Among the most important sources of epigenetic silencing in humans is the Human Silencing Hub (HUSH) complex, consisting of three proteins: Periphilin, TASOR and MPP8 (11). In the current model of HUSH-dependent repression HUSH spreads histone H3 lysine 9 trimethylation (H3K9me3), a transcriptionally repressive mark, by recruiting the H3K9 methyltransferase SETDB1 and its stabilizing factor ATF7IP to existing H3K9me3 marks via MPP8, which binds both H3K9me3 and ATF7IP. Here, we report the crystal structure of a Periphilin-TASOR minimal core complex and identify the key physicochemical properties of Periphilin necessary for HUSH complex assembly and epigenetic silencing. The Periphilin C-terminal region directs HUSH complex assembly by dimerizing and binding a single TASOR molecule through α-helical coiled-coil interactions.

Thus, a crystal structure of a Periphilin fragment spanning residues 292–367 bound to a TASOR fragment spanning residues 1014–1095 was determined using the single anomalous dispersion (SAD) phasing method, with bromine as the anomalous scatterer. The structure contains two Periphilin molecules and a single TASOR molecule. The Periphilin fragments form helical hairpins with a mixture of α-helix and 310-helix secondary structure. The two Periphilin hairpins pack against each other via a 118 Å2 hydrophobic interface formed by the hydrophobic side chains of Leu326, Leu333 and Ile337. The resulting Periphilin homodimer has twofold symmetry. The TASOR molecule forms two α-helices that wrap around the outer surfaces of the Periphilin dimer. The TASOR helices add a third helix to each Periphilin helical hairpin to form two three-helix coiled-coils. Unusually, however, each Periphilin subunit binds to a different TASOR sequence (residues 1014–1052 and 1072–1093, respectively) with an identical binding surface. Notably residues 1055–1071 of TASOR, between the two Periphilin-binding segments, are disordered, but these 17 residues could easily span the 35–40 Å trajectory needed to connect residues 1054 and 1072 in the Periphilin-TASOR complex. The 2:1 stoichiometry of the Periphilin-TASOR core complex was confirmed in solution by size-exclusion chromatography coupled with multiangle light scattering (SEC-MALS) and non-denaturing mass spectrometry.

>MGSSHHHHHHSQENLYFQSQLTTRSKAIASKTKEIEQVYRQDCETFGMVVKMLIEKDPSLEKSIQFALRQNLHEIGERCVEELKHFIAEYDTST[2x];> MSETTERTVLGEYNLFSRKIEEILKQKNVSYVSTVSTPIFSTQEKMKRLSEFIYSKTSKAGVQEFVDGLHEKLNTIIIKASAK> SAGAGSHCQKTSLRVNFEDIGWDSWIIAPKEYEAYECKGGCFFPLADDVTPTKHAI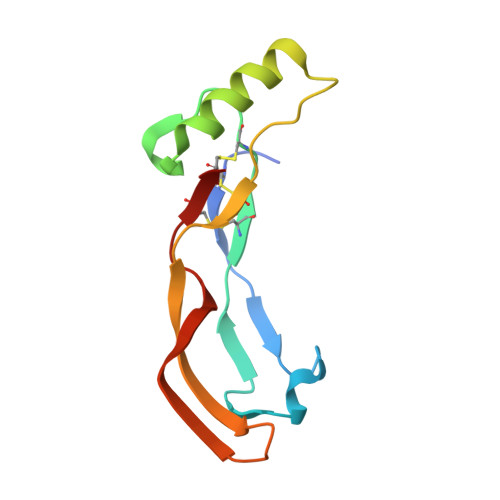VQTLVHLKFPTKVGKACCVPTKLSPISVLYKDDMGVPTLKYHYEGMSVAECGCR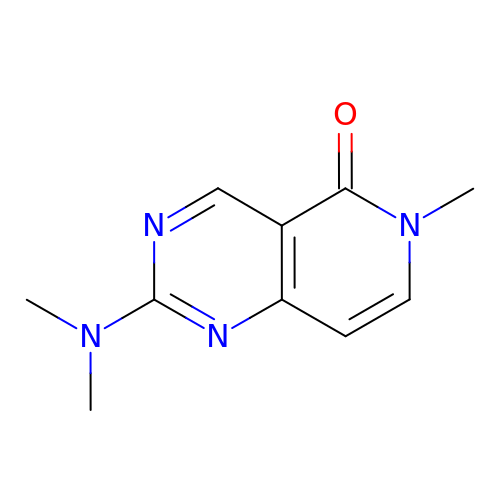2-(dimethylamino)-6-methyl-pyrido[4,3-d]pyrimidin-5-one | C10 H12 N4 O | YKBGUFTWJZHVCT-UHFFFAOYSA-N>SNAPNPISIPIDLSQAGSVVEKEVKIEESWSYHLILQFAVHDRKEDGGLDGKRVW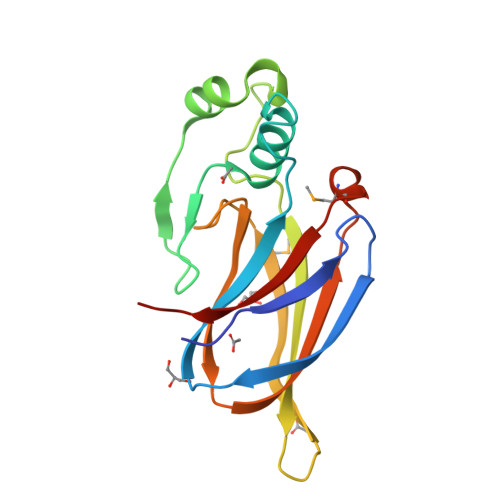KFLGFNSYDPRDGKQVGYVDYRLAKSELGDLIDETYDCDGTVVPIKITIHQINQDNTKKLIADNLYMTKGNGSGAYTRDITTISLDKGKYIFRIENIEAFSEMIGRKVDFTIYINKRDK[2x]> MIVLFVDFDYFYAQVEEVLNPSLKGKPVVVCVFSGRFEDSGAVATANYEARKFGVKAGIPIVEAKKILPNAVYLPMRKEVYQQVSSRIMNLLREYSEKIEIASIDEAYLDISDKVRDYREAYNLGLEIKNKILEKEKITVTVGISKNKVFAKIAADMAKPNGIKVIDDEEVKRLIRELDIADVPGIGNITAEKLKKLGINKLVDTLSIEFDKLKGMIGEAKAKYLISLARDEYNEPIRTR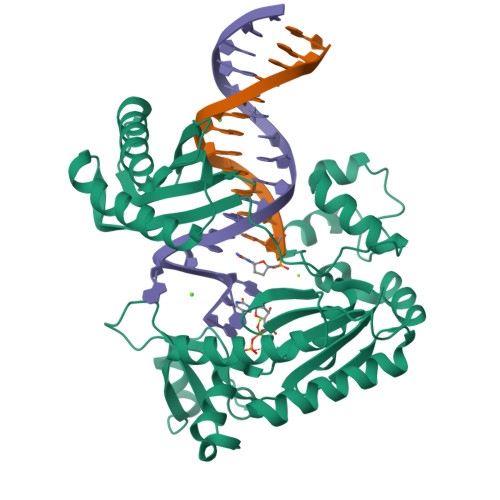VRKSIGRIVTMKRNSRNLEEIKPYLFRAIEESYYKLDKRIPKAIHVVAVTEDLDIVSRGRTFPHGISKETAYSESVKLLQKILEEDERKIRRIGVRFSKFIE>MHHHHHHSSGLVPRGSHMSHVPPHVPFELSGAELRDAIVQYATNPIYHDNLDWLNHDNPYRRQLRPQVLPHLDYDKVPGRENILNYASLAVQRLLTSVYEADLVFFPKSGLKGKEEDFRAFYSPANRALGERIRPALERYAFGFLDDEVETSGTWTAQSLDAYLDSLDTAGGAEQSPVEKAILGSADRERAARMWLVQFAPDFLSEASPMMRNVLGYYGPAQSEWFKVVIDEYGYGVHDTKHSTLFERTLESVGLESDLHRYWQYYLNSSLLLNNYFHYLGKNHELFFRYVGALYYTESSLVDFCRRADHLLREVFGDTVDTTYFTEHIHIDQHHGRMARE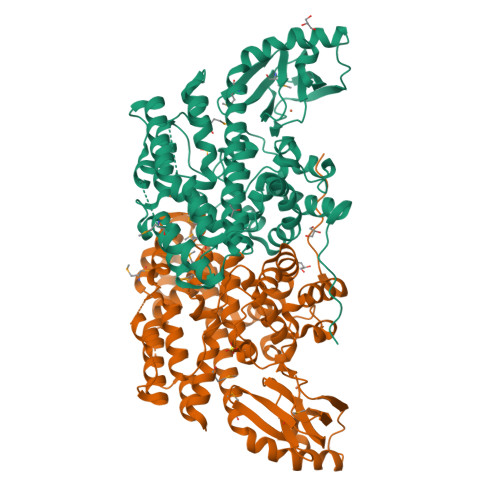KIIKPLVEAHGDGIIPEIVRGIEEYRVLLEIGDFDFSEQIAWMDAQPELKKLHDPVFEGLKQGKVDAPVAHLVEPRGELSNTHCHDGDELCHIVSGTMRFESGLGSSLTLQAGEGVVIKRNRLHGANIESDECVYEIHSVGDYRKCL[4x]PNGM-1 is derived from a metagenomic library from deep-sea sediments that predate the antibiotic era. PNGM-1 has both MBL and tRNase Z activities and is considered to be the evolutionary origin of B3 MBLs. The wild-type of PNGM-1 has two MBSs in its substrate-binding pocket, and each is occupied by a zinc ion. The zinc ion in the first MBS (Zn1) is coordinated by the residues His91, His93, His188, and Asp210; the zinc ion in the second MBS (Zn2), by Asp95, His96, His279, and Asp210.

His91 and His93 coordinate the zinc ion at Zn1, whereas His96 and His279 coordinate that at Zn2. In the crystal structures of the H96A and H279A variants, the electron density of the zinc ion at Zn2 is markedly lower compared to that in the wild-type structure, indicating that either a water molecule with full occupancy or a zinc ion with half occupancy is present in this site. In H96A, even though electron density exists for the zinc ion at Zn2, the density is weak and noisy, implying weak binding of the metal ion. Among all the variants, H91A and H96A exhibit the lowest metal occupancy. From a structural viewpoint, the substitution of His91 and His96 by alanine markedly weakens the metal binding affinity for Zn1 and Zn2, respectively, compared to that of the wild-type and the remaining variants. The residues His91 and His96 are buried in the substrate-binding pocket of PNGM-1. In the structures of all PNGM-1 variants, except in that of H96A, the electron density corresponding to the catalytic water remains despite the complete or partial loss of a zinc ion. Each MBS of PNGM-1 is formed by four metal-coordinating residues, and the substitution of only one of these residues dramatically reduces the metal binding affinity of the enzyme.

>[4x]STGIAPKRYVYYPGSEELGPDEIRVIACGTGMPTARRAQAAAAWVVELGNGDKFIVDIGSGSMANIQSLMIPANYLTKIFLTHLHTDAWGDLVSMWAGGWTAGRTDPLEVWGPSGSREDMGTKYAVEHMLKAYNWDYMTRAVTINPRPGDINVHEFDYRALNEVVYQENGVTFRSWPCIHAGDGPVSFALEWNGYKVVFGGDTAPNIWYPEYAKGADLAIHECWMTSDQMMTKYNQPAQLALRINLDFHTSAQSFGQIMNMVQPRHAVAYHFFNDDDTRYDIYTGVRENYAGPLSMATDMMVWNITRDAVTERMAVSPDHAWDVAGPSEDLAPDRNRASEYTQYILDGRLNVDEANAHWKQEFMG>[4x]MRPARALIDLQALRHNYQLAREVTGAKALAVIKADAYGHGAVRCAQALEAEADGFAVAC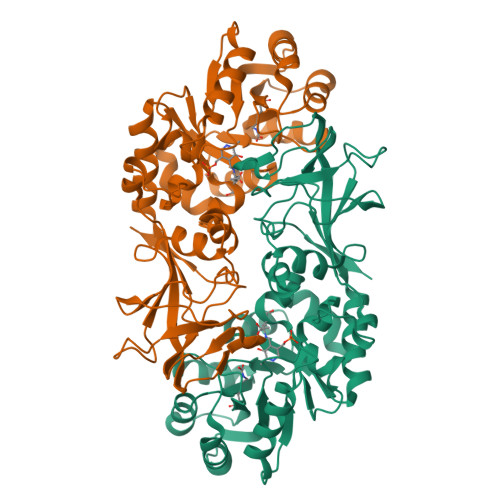IEEALELRAAGIRAPILLLEGFFEADELPLIVEHDFWCVVHSLWQLDAIEQARLAKPIHVWLKLDSGMHRVGLHPNDYKAAYQRLQASANVAKIVLMSHFARADELDCTRSVEQVAVFLGARADLTAEISLRNSPAVLGWPRVPSDWVRPGLMLYGSSPFDEPQATASRLQPVMTLESKVICVRELPAGEPVGYGARFITPKPMRIGVVAMGYADGYPRQAPTGTPVFVDGVRSQLLGRVSMDMLCIDLTDVPQAGLGSTVELWGKNILASEVATAADTIPYQIFCNLKRVPRLYSGN8-(azaindolyl)-benzoazepinone 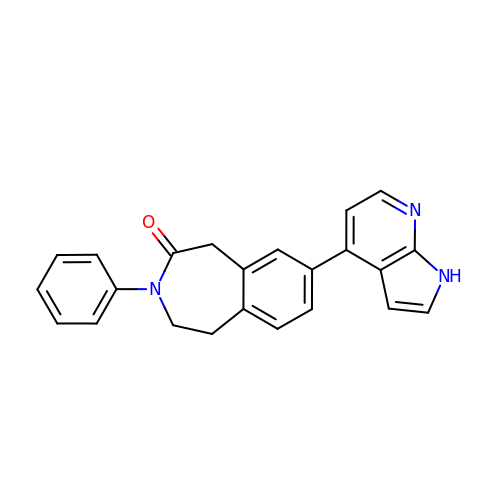| C23 H19 N3 O | ZOBOJXLVNHCFCC-UHFFFAOYSA-N> XXXXXXXXXXXXXXXXXXXXXXXXXXXXXXXXXXXXXXXXXXXMLSSARRLLATVAEQRALAKADAPAAAAQLRARAGLASVSCCGSTTATITTRLGATGSWRHMSSAADSTSSSSSSSSSQQQQPPAQQQQQPEASTSSAAASSPDGPMSEVVQQLTKASPTGRLLDLFTPSQQQIQTLQRSRGPGRGSRSGT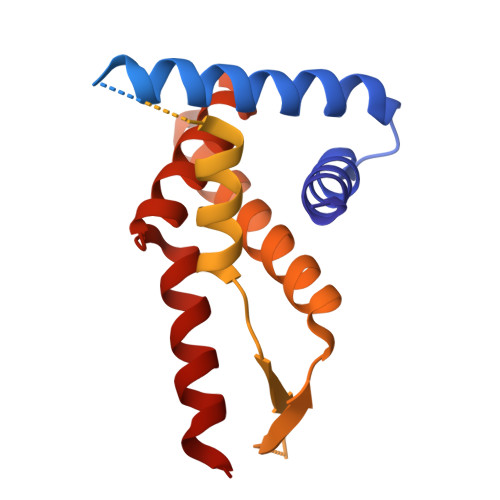GPAGPAAGTGVQAAEAAAPLTADSDVLEVLMRAVDNCKPLMKVIQSKAGTRVVYQPRPLNPDQSTNFAVKWILQAAQKRRAGAKGVAGAASMAEALAVELLLAAQRKGGARARRDEVHKLALDNRANLRR>MHHHHHHENLYFQGADQGSAEEVSVEELKAIQLRTTNEATGEKRFGSARAIIEDLTIYKSDGTTLAEKPLIKSGEEVTFDFTILASEEIKDIALGISMSKAQGGDIW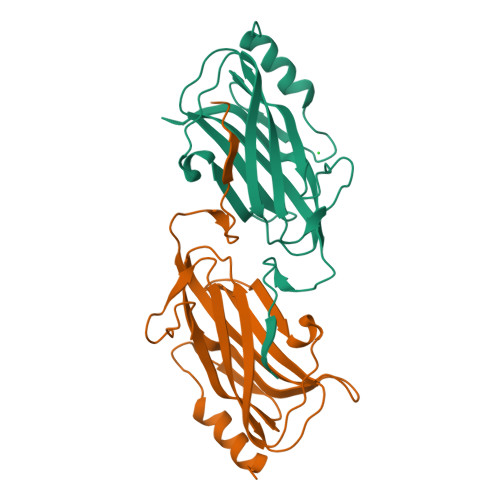GDSNIGAGSAITLRPGRQRIVYKATLPINSGDYLIHCGLAKVGNGDREELDQRRPMMKVKFWSARELGGVIHAPLKIISNGES[3x]>MKKIHTDK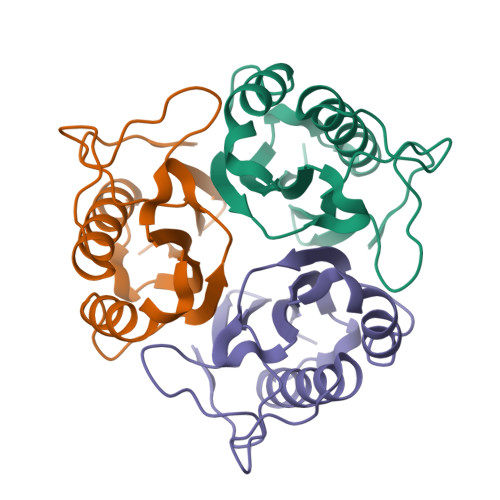APAAIGPYVQGKIVGNLLFASGQVPLSPETGQVIGTTIEEQTQQVLKNISAILTEAGTDFDHVVKTTCFLSDIDDFVPFNEVYATAFKSDFPARSAVEVARLPKDVKIEIEVIAELI[9x]> SNAMNNHQTPQATSPLAAWLCYLEHLHSQPIELGLERVKQVAERLDLLKPAPKIFTVAGTNGKGTTCCTLEAILLAAGLRVGVYSSPHLLRYTERVRIQGQELSEAEHSHSFAQIEAGRGDISLTYFEFGTLSALQLFKQAKLDVVILEVGLGGRLDATNIVDSDVAAITSIALDHTDWLGYDRESIGREKAGVFRGGKPAVVGEPDMPQSIADVAAELGAQLYRRDVAWKFSQQEPFDQQEPVDQQINGWHWQCGERQLTGLPVPNVPLANAATALAVLHYSELPLSDEAIRQGLQAASLPGRFQVVSEQPLLILDVAHNPHAARYLVNRLAQVINPVNASKQGKVRAVVGMLSDKDIAGTLACLSERVDEWYCAPLEGPRGASAGQLAEHLVSARQFSDVETAWRQAMQDADTQDVVIVCGSFHTVAHVMAA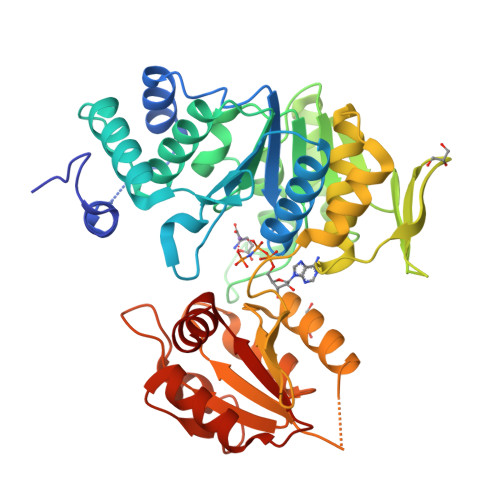LHL> MGDSEEVNERVKQLAEKAKEATDKEEVIEIVKELAELAKQSTDPNVVAEIVYQLAEVAEHSTDPELIKEILQEALRLAEEQGDEEL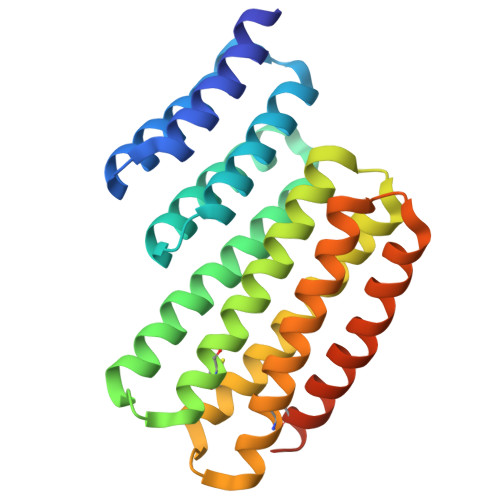AEAARLALKAARLLEEARQLLSKDPENEAAKECLKAVRAALEAALLALLLLAKHPGSQAAQDAVQLATAALRAVEAACQLAKQYPNSDIAKKCIKAASEAAEEASKAAEEAQRHPDSQKARDEIKEASQKAEEVKERCERAQEHPNAGWLEHHHHHH> MGSSHHHHHHGSNAIISPDYYYVLTVAGQSNAMAYGEGLPLPDREDAPHPRIKQLARFAHTHPGGPSCHFNDIIPLTHCPHDVQDMQSYHHPLATNHQTQYGTVGQALHIARKLLPFIPDNAGILIVPCCRGGSAFTAGSEGTYSERHGASHDACRWGT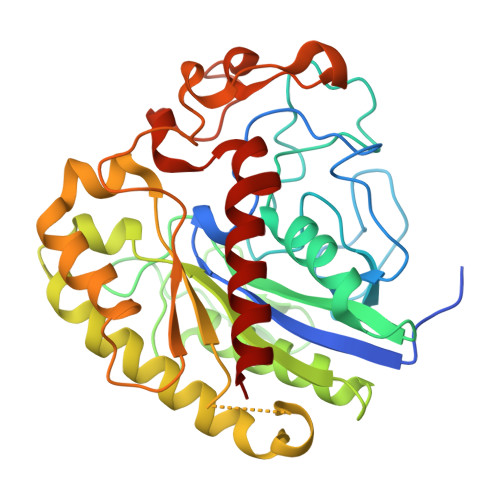DTPLYQDLVSRTRAALVKNPQNKFLGVCWMQGEFDLMTSDYASHPQHFNHMVEAFRRDLKQYHSQLNNITDAPWFCGDTTWYWKENFPHAYEAIYGNYQNNILANIIFVDFQQQGARGLTNAPDEDPDDLSTGYYGSAYRSPENWTTALRSSHFSSAARRGIISDRFVEAILQFWRER1,1,1,3,3,3-hexafluoro-2-[2-fluoro-4'-({4-[(pyridin-4-yl)methyl]piperazin-1-yl}methyl)[1,1'-biphenyl]-4-yl]propan-2-ol | C26 H24 F7 N3 O | 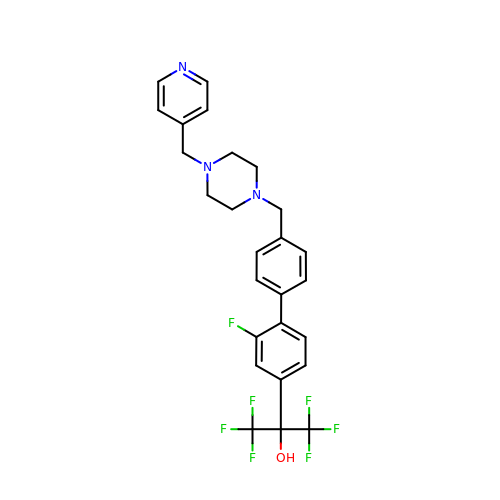KVHKWAZUPPBMLL-UHFFFAOYSA-N> 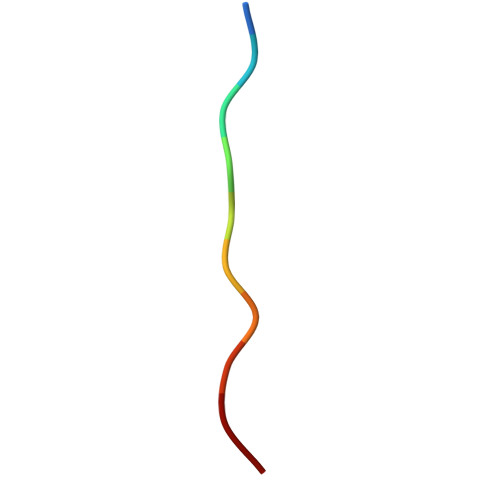GGGGGGGGGG>AQCEATIESNDAMQYDLKEMVVDKSCKQFTVHLKHVGKMAKSAMGHNWVLTKEADK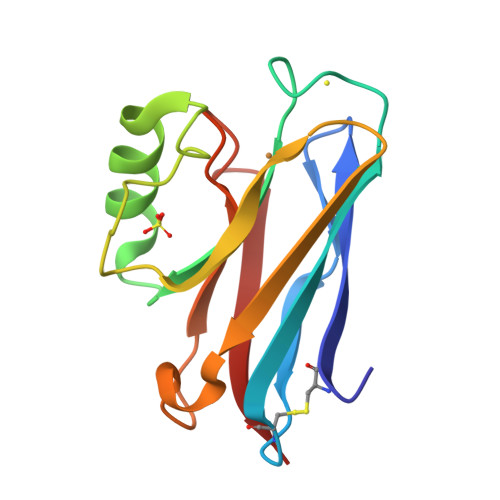EGVATDGMNAGLAQDYVKAGDTRVIAHTKVIGGGESDSVTFDVSKLTPGEAYAYFCSFPGHWAMMKGTLKLSN[2x]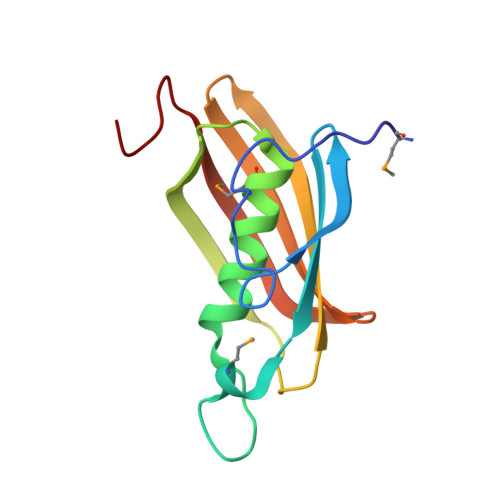> MIPVEQRTHKLTSRILVGKPILIKEGYAEVELETIDEMKVDEKGLVHGGFTFGLADYAAMLAVNEPTVVLGKAEVRFTKPVKVGDKLVAKAKIIEDLGKKKIVEVKVYREEEVVLEGKFYCYVLEKHVLDN>[10x]DVQPETCRPSAASGNYFPQYPEYAIETARLRTFEAWPRNLKQKPHQLAEAGFFYTGVGD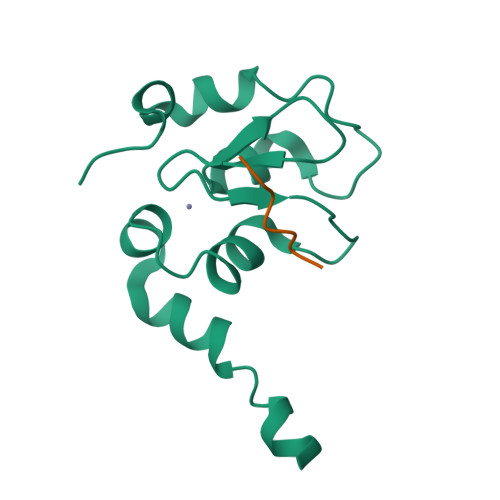RVRCFSCGGGLMDWNDNDEPWEQHALWLSQCRFVKLMKGQLYIDTVAAKPVLAEEKEESTSIGGD;>[10x]SRPPFISLNERR>[4x]AYMFSDRSTSLSIEEERFLDAAEYGNIPVVRKMLEECHSLNVNCVDYMGQNALQLAVANEHLEITELLLKKENLSRVGDALLLAISKGYVRIVEAILSHPAFAEGKRLATSPSQSELQQDDFYAYDEDGTRFSHDVTPIILAAHCQEYEIVHTLLRKGARIERPHDYFCKCNDCNQKQKHDSFSHSRSRINAYKGLASPAYLSLSSEDPVMTALELSNELAVLANIEKEFKNDYKKLSMQCKDFVVGLLDLCRNTEEVEAILNGDVETLQSGDHGRPNLSRLKLAIKYEVKKFVAHPNCQQQLLSIWYENLSGLRQQTMAVKFLVVLAVAIGLPFLALIYWFAPCSKMGKIMRGPFMKFVAHAASFTIFLGLLVMNAADRFEGTKLLPNETSTDNAKQLFRMKTSCFSWMEMLIISWVIGMIWAECKEIWTQGPKEYLFELWNMLDFGMLAIFAASFIARFMAFWHASKAQSIIDANDTLKDLTKVTLGDNVKYYNLARIKWDPSDPQIISEGLYAIAVVLSFSRIAYILPANESFGPLQISLGRTVKDIFKFMVIFIMVFVAFMIGMFNLYSYYIGAKQNEAFTTVEESFKTLFWAIFGLSEVKSVVINYNHKFIENIGYVLYGVYNVTMVIVLLNMLIAMINSSFQEIEDDADVEWKFARAKLWFSYFEEGRTLPVPFNLVPSPKSLFYLLLKLKKWISELFQGHKKGFQEDAEMNKINEEKKLGILGSHEDLSKLSLDKKQVGHNKQPSIRSSEDFHLNSFNNPPRQYQKIMKRLIKRYTTQAQIDKESDEVNEGELKEIKQDISSLRYELLEEKSQNTEDLAELIRELGEKLSMEPNQEETNR

The mammalian TRPC subfamily consists of seven transmembrane proteins (TRPC1-7) that have been proposed to form non-selective cation channels in various cell types. TRPC6 and its most close homologs TRPC3 and TRPC7 are unique among the TRPCs in that they can be directly activated by second messenger diacylglycerol (DAG), a product of phospholipase C action. TRPC6-mediated cation influx regulates physiological function of pulmonary endothelial cells, smooth muscle cells and glomerular podocytes, whereas TRPC6 hyperactivity has been implicated in maladaptive tissue and organ remodeling. In this study, we present two high-resolution cryo-EM structures of antagonist- and agonist-bound human TRPC6 in lipidic nanodiscs.

Furthermore, because TRPC6 V867T/L868T, like WT, responded to both AM-0883 and OAG but exhibited much higher channel activity than WT, the double mutant appeared to be an ideal variant for us to investigate the more activated state of TRPC6. We found a clear non-protein density at each subunit interface that represents the agonist AM-0883, which consists of a chloro-indole, a piperidine and a benzodioxin, and occupies a groove between S6 of one subunit and the pore helix of the adjacent subunit. The agonist forms hydrophobic interactions with Phe675 and TRP680 on the pore helix and Tyr705, Val706 and Val710 on S6. There are also possible hydrophilic interactions between the indole ring and Glu672 and Asn702. We tested whether mutations around this region would affect the potency of the agonist and found that mutations F675A, W680A, N702A, Y705A and V710A almost completely abolished the channel activity in the presence of the agonist AM-0883, whereas mutations E672A and V706A showed a 35-fold and 20-fold increase in agonist EC50, respectively. Notably, the AM-0883-binding site faces membrane lipids and is occupied by one of the outer leaflet lipids in the antagonist-bound structure, and therefore constitutes a likely location for DAG-binding at the outer leaflet. However, similar to the antagonist-bound structure of TRPC6 (Δ2–72), the agonist-bound structure of TRPC6 (Δ2–72) V867T/L868T also possesses a closed ion channel pore. Instead, the presence of the agonist seems to tilt the extracellular half of S6 away from the pore and pushes S6 toward the intracellular side. Because S6 is tightly packed against S1-S4 of the adjacent subunit, the movement of S6 is accompanied by a concurrent tilting and downward movement of S1-S4 as well as the S4-S5 linker.The WWE domain is a relatively under-researched domain found in twelve human proteins and characterized by a conserved tryptophan-tryptophan-glutamate (WWE) sequence motif. Six of these WWE domain-containing proteins also contain domains with E3 ubiquitin ligase activity. Here, we present novel crystal structures of the HUWE1, TRIP12, and DTX1 WWE domains in complex with PAR building blocks and their analogs, thus enabling a comprehensive analysis of the PAR binding site structural diversity. A highly conserved feature in all determined structures is the recognition and therefore the interactions involving the adenine ring of the ligands.

Generally, the dissociation constants of our ligands for HUWE1 were higher, apart from iso-ADPr, which was determined to be the weakest (Kd = 132 µM, compared to ADPr, ATP, 2F-ATP (1) and 2’F-ATP (2) with Kd’s of 15 µM to 59 µM). Based on the high binding affinity of the HUWE1 WWE domain to 2’F-ATP (15 µM, ~2.5-fold higher than for ADPr), we solved the co-crystal structure with 2’F-ATP revealing a different binding mode compared to ADPr. The fluorine group of 2’F-ATP overlays with the pyrazole nitrogen of the adenine backbone in the ADPr binding site. The ligand mainly interacts with a network of water molecules and a hydrogen bond of a ribose oxygen to Gln1667, as well as π-π interactions with the conserved Trp1619 aromatic sidechain. Overall, the binding mode of the phthalimide scaffold overlays with the adenine-backbone of the natural substrate-derived ADPr and the 2’F-ATP (2) molecule, suggesting competitive behavior.

>[4x]GQSNSNNWRWFDDRSGRWCSYSASNNSTIDSAWKSGETSVRFTAGRRRYTVQFTTMVQVNEETGNRRPVMLTLLRVPRLNKNSKNSNGQEL>[2x]MKSVVNDTDGIVRVAESVIPEIKHQDEVRVKIASSGLCGSDLPRIFKNGAHYYPITLGHEFSGYIDAVGSGVDDLHPGDAVACVPLLPCFTCPECLKGFYSQCAKYDFIGSRRDGGFAEYIVVKRKNVFALPTD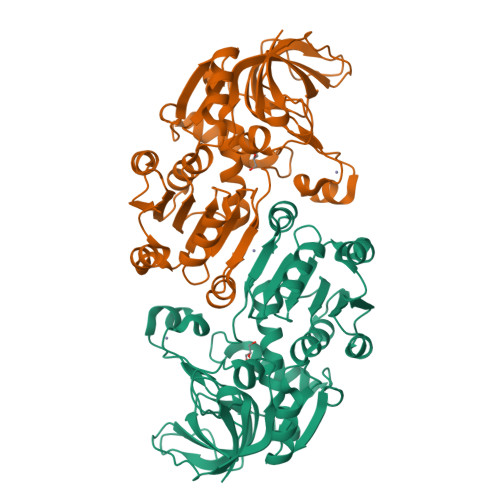MPIEDGAFIEPITVGLHAFHLAQGCENKNVIIIGAGTIGLLAIQCAVALGAKSVTAIDISSEKLALAKSFGAMQTFNSSEMSAPQMQSVLRELRFNQLILETAGVPQTVELAVEIAGPHAQLALVGTLHQDLHLTSATFGKILRKELTVIGSWMNYSSPWPGQEWETASRLLTERKLSLEPLIAHRGSFESFAQAVRDIARNAMPGKVLLIP> GSSTPDAVDKYLETPGDENEHAHFQKAKERLEAKHRERMSQVMREWEEAERQAKNLPKADKKAVIQHFQEKVESLEQEAANERQQLVETHMARVEAMLNDRRRLALENYITALQAVPPRPHHVFNMLKKYVRAEQKDRQHTLKHFEHVRMVDPKKAAQIRSQVMTHLRVIYERMNQSLSLLYNVP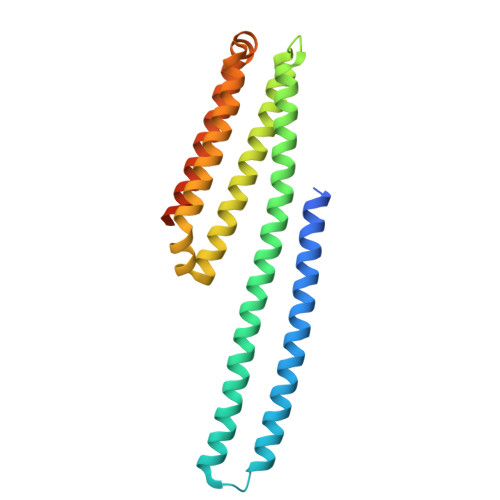AVAEEIQDEVDELLQKEQNYSDDVLANMISEPRISYGNDASGRGLVPR> MKLFNRYRVALLSALPLALCALSAAAQVVQEYEYAPDRIYQVRTGLGITTQVELSPNEKILDYSTGFTGGWELTRRENVFYLKPKNVDVDTNMMIRTATHSYILELKVVATDWQRLEQAKQAGVQYKVVFTYPKDTSFNNVADADTSKNGPLLNAKILKDRRYYYDYDYATRTKKSWLIPSRVYDDGKFTYINMDLTR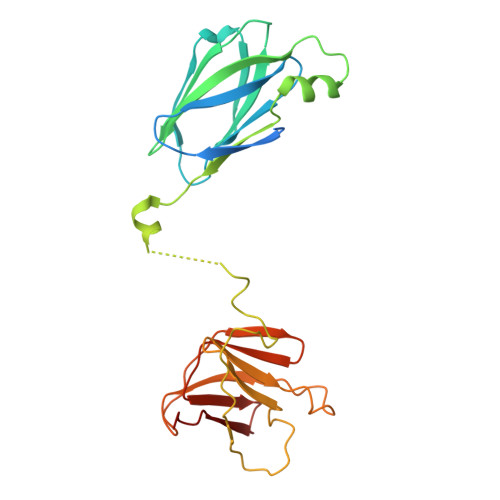FPTGNFPAVFAREKEHAEDFLVNTTVEGNTLIVHGTYPFLVVRHGDNVVGLRRNKQK>MDVLTKLLNRRFLPTI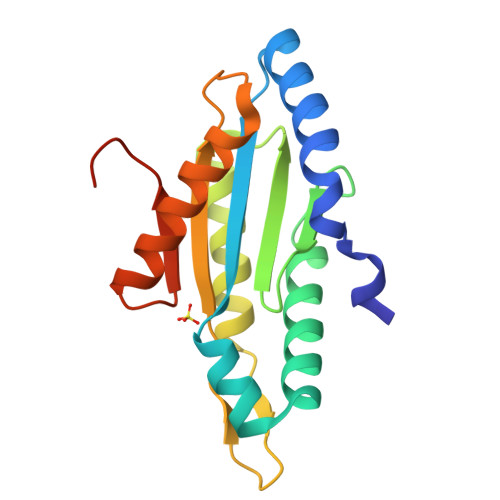FKREIAHANRTGTPLSVLIIDVDKFKEINDTWGHNTGDEILRKVSQAFYDNVRSSDYVFRYGGDEFIIVLTEASENETLRTAERIRSRVEKTKLKAANGEDIALSLSIGAAMFNGHPDYERLIQIADEALYIAKRRGRNRVELWKASLLEHHHHHH[2x]>MTDTTNSIKHVISPLARQTLQDRDLTRPVAGKRPIRLLPWLQVVKIGGRVMDRGADAILPLVEELRKLLPEHRLLILTGAGVRARHVFSVGLDLGLPVGSLAPLAASEAGQNGHILAAMLASEGVSYVEHPTVADQLAIHLSATRAVVGSAFPPYHHHEFPGSRIPPHRADTGAFLLADAFGAAGLTIVENVDGIYTADPNGPDRGQARFLPETSATDLAKSEGPLPVDRALLDVMAT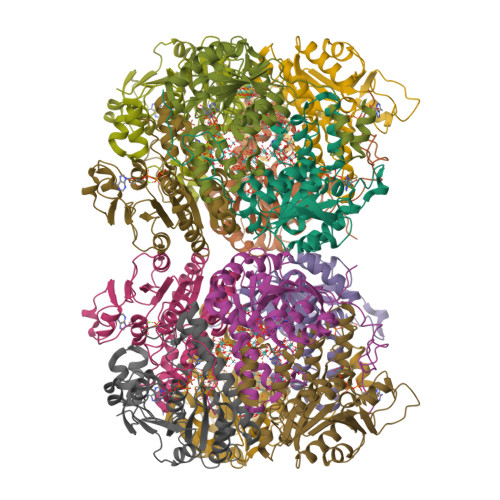ARHIERVQVVNGLVPGRLTAALRGEHVGTLIRTGVRPA[6x];>MANSTAELEELLMQRSLTDPQLQAAAAAAADFRILPDATVIKIGGQSVIDRGRAAVYPLVDEIVAARKNHKLLIGTGAGTRARHLYSIAAGLGLPAGVLAQLGSSVADQNAAMLGQLLAKHGIPVVGGAGLSAVPLSLAEVNAVVFSGMPPYKLWMRPAAEGVIPPYRTDAGCFLLAEQFGCKQMIFVKDEDGLYTANPKTSKDATFIPRISVDEMKAKGLHDSILEFPVLDLLQSAQHVREVQVVNGLVPGNLTRALAGEHVGTIITAS[6x]(2R)-2-[(E)-[2-methyl-3-oxidanyl-5-(phosphonooxymethyl)pyridin-4-yl]methylideneamino]-3-oxidanyl-propanoic 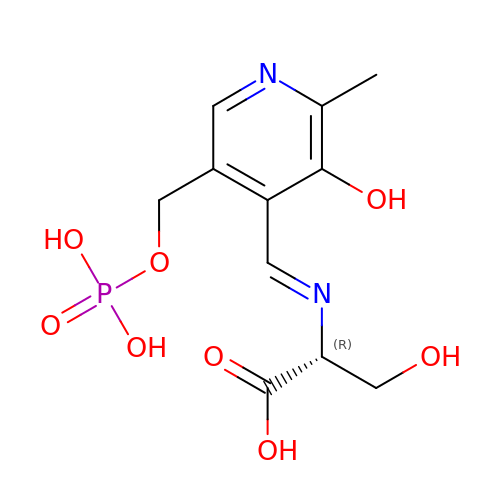acid | C11 H15 N2 O8 P | ZTQZHYMXYBDMIL-RZTFRGLUSA-N> IVGGQECKDGECPWQALLINEENEGFCGGTILSEFYILTAAHCLYQAKRFKVRVGDRNTEQEEGGEAVHEVEVVIKHNRFTKETYDFDIAVLRLKTPITFRMNVAPACLPERDWAESTLMTQKTGIVSGFGRTHEKGRQSTRLKMLEVPYVDRNSCKLSSSFIITQNMFCAGYDTKQEDACQGDSGGPHVTR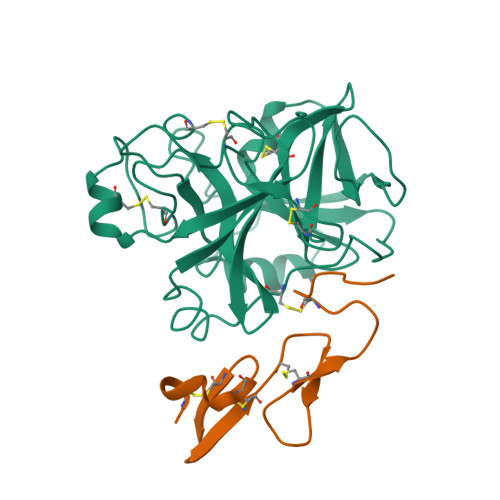FKDTYFVTGIVSWGEGCARKGKYGIYTKVTAFLKWIDRSMKTRGLPKAKSHAPEVVITSSPLK;> YKDGDQCETSPCQNQGKCKDGLGEYTCTCLEGFEGKNCELFTRKLCSLDNGDCDQFCHEEQNSVVCSCARGYTLADNGKACIPTGPYPCGKQTLER>GPMGKELKIGVPLRVSYKEFVSQIRGTENMFKGFCIDVFTAAVNLLPYAVPVKFIPYGNGKENPSYTHMVEMITTGNFDGVVGDVAIVTNRTKIVDFTQPYAASGLVVVAPGGTPIKGIESLRERDDPIGYQVGSFAESYLRNELNISESRLVPLGTPEAYAKALKDGPSKGGVAAIVDERPYVELFLSSNCAYRIVGQEFTKSGWGFAFPRDSPLAIDLSTAILELAENGDLQRIHDKWLM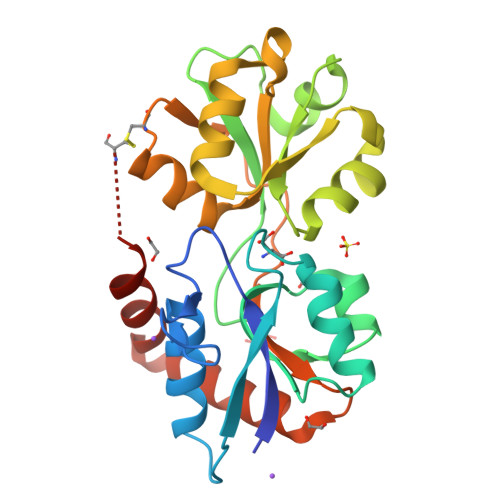KNACT[2x]> GSKQKEAIKVYLELLEVHSRVLKALIEQIKLFIELIMEPDED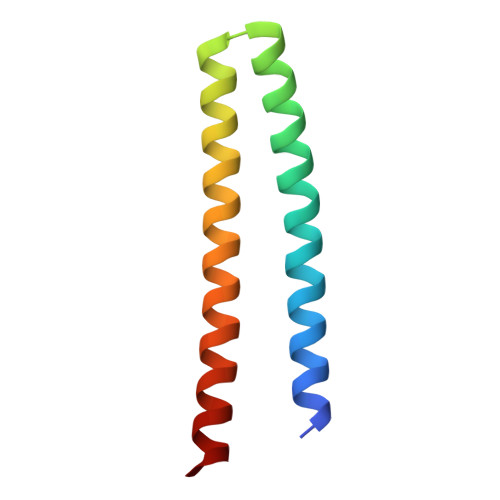LADKVRKSSEELKKIIKEVEKILRKVDDILEKVKS>[2x]TIPGNFAAYHELWRNAFQEIMNDPRHQL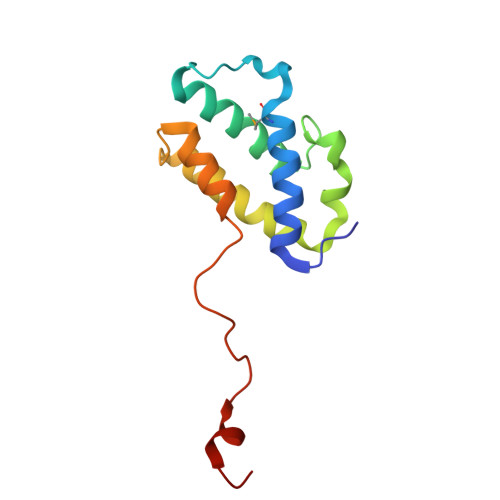HRNDVEYKKIHAIRTVLDDYTKGGNTWWAKFRRIFTFHWNRHHVKVVDDIVKEIDAGNYTTSRALVDRLDNLAISLGSKLNPKGTLKEQIGFIK>[2x]MVLYFIGLGLYDERDITVKGLEIAKKCDYVFAEFYTSLMAGTTLGRIQKLIGKEIRVLSREDVELNFENIVLPLAKENDVAFLTPGDPLVATTHAELRI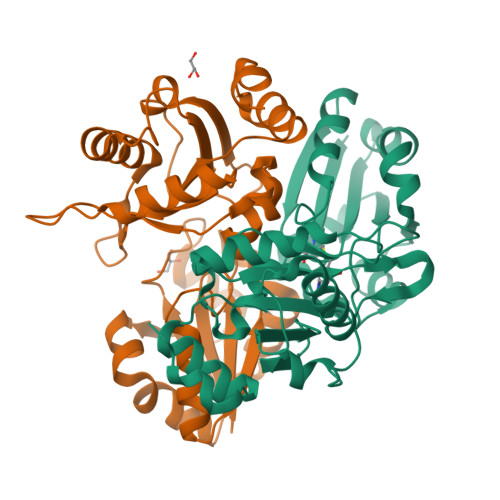RAKRAGVESYVIHAPSIYSAVGITGLHIYKFGMSATVAYPEGNWFPTSYYDVIKENAERGLHTLLFLDIKAEKRMYMTANEAMELLLKVEDMKKGGVFTDDTLVVVLARAGSLNPTIRAGYVKDLIREDFGDPPHILIVPGKLHIVEAEYLVEIAGAPREILRVNV5-methyl-2-phenyl-2,4-dihydro-3H-pyrazol-3-one 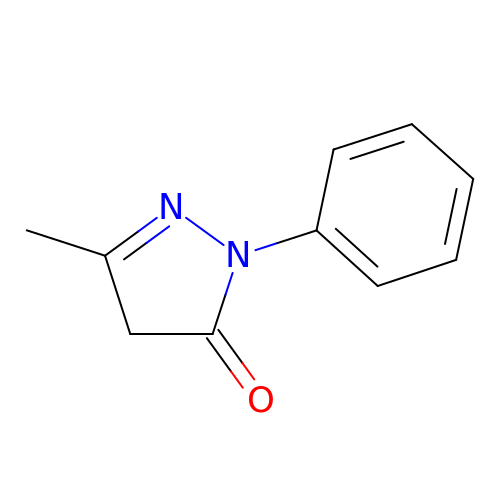| C10 H10 N2 O | QELUYTUMUWHWMC-UHFFFAOYSA-N>[7x]EVKQENRLLNESESSSQGLLGYYFSDLNFQAPMVVTSSTTGDLSIPSSELENIPSENQYFQSAIWSGFIKVKKSDEYTFATSADNHVTMWVDDQEVINKASNSNKIRLEKGRLYQIKIQYQRENPTEKGLDFKLYWTDSQNKKEVISSDNLQLPELKQKSSNSRKKRSTSAGPTVPDRDNDGIPDSLEVEGYTVDVKNKRTFLSPWISNIHEKKGLTKYKSSPEKWSTASDPYSDFEKVTGRIDKNVSPEARHPLVAAYPIVHVDMENIILSKNEDQSTQNTDSQTRTISKNTSTSRTHTSEVHGNAEVHASFFDIGGSVSAGFSNSNSSTVAIDHSLSLAGERTWAETMGLNTADTARLNANIRYVNTGTAPIYNVLPTTSLVLGKNQTLATIKAKENQLSQILAPNNYYPSKNLAPIALNAQDDFSSTPITMNYNQFLELEKTKQLRLDTDQVYGNIATYNFENGRVRVDTGSNWSEVLPQIQETTARIIFNGKDLNLVERRIAAVNPSDPLETTKPDMTLKEALKIAFGFNEPNGNLQYQGKDITEFDFNFDQQTSQNIKNQLAELNATNIYTVLDKIKLNAKMNILIRDKRFHYDRNNIAVGADESVVKEAHREVINSSTEGLLLNIDKDIRKILSGYIVEIEDTEGLKEVINDRYDMLNISSLRQDGKTFIDFKKYNDKLPLYISNPNYKVNVYAVTKENTIINPSENGDTSTNGIKKILIFSKKGYEIG;>MNEHYTESDIKRNHKTEKNKTEKEKFKDSINNLVKTEFTNETLDKIQQTQDLLKKIPKDVLEIYSELGGEIYFTDIDLVEHKELQDLSEEEKNSMNSRGEKVPFASRFVFEKKRETPKLIINIKDYAINSEQSKEVYYEIGKGISLDIISKDKSLDPEFLNLIKSLSDDSDSSDLLFSQKFKEKLELNNKSIDINFIKENLTEFQHAFSLAFSYYFAPDHRTVLELYAPDMFEYMNKLEKGGFEKISESLKKEGVEKDRIDVLKGEKALKASGLVPEHADAFKKIARELNTYILFRPVNKLATNLIKSGVATKGLNVHGKSSDWGPVAGYIPFDQDLSKKHGQQLAVEKGNLENKKSITEHEGEIGKIPLKLDHLRIEELKENGIILKGKKEIDNGKKYYLLESNNQVYEFRISDENNEVQYKTKEGKITVLGEKFNWRNIEVMAKNVEGVLKPLTADYDLFALAPSLTEIKKQIPQKEWDKVVNTPNSLEKQKGVTNLLIKYGIERKPDSTKGTLSNWQKQMLDRLNEAVKYTGYTGGDVVNHGTEQDNEEFPEKDNEIFIINPEGEFILTKNWEMTGRFIEKNITGKDYLYYFNRSYNKIAPGNKAYIEWTDPITKAKINTIPTSAEFIKNLSSIRRSSNVGVYKDSGDKDEFAKKESVKKIAGYLSDYYNSANHIFSQEKKRKISIFRGIQAYNEIENVLKSKQIAPEYKNYFQYLKERITNQVQLLLTHQKSNIEFKLLYKQLNFTENETDNFEVFQKIIDEK[2x]

Following assembly, the anthrax protective antigen (PA) forms an oligomeric translocon that unfolds and translocates either its lethal factor (LF) or edema factor (EF) into the host cell. The toxin functions as a binary A2B toxin, with enzymatic A factors, lethal factor (LF, 91 kDa) and edema factor (EF, 89 kDa), and a cell binding B factor, protective antigen (PA, 83 kDa). Within the endosomal compartment, the acidic environment induces a conformational change in the PA, resulting in the formation of a β-barrel channel that can insert itself into the endosomal membrane. The first α helix and β strand of LF and EF unfold and dock into a deep amphipathic cleft, called the α clamp, which resides at the interface of two PA monomers.

The available space on the heptameric PA channel for EF binding can only accommodate up to three EF molecules due to steric hindrance. Indeed, 2D classification of cryo-EM images of PA channel bound with EF showed that the EF binding varies in different classes, suggesting that the space is not fully occupied. Therefore, we used a symmetry expansion method in Relion for 3D classification and were able to resolve the asymmetrically attached EF. Unlike LF, all the domains of EF are well resolved in our channel complex structures. Upon PA binding, these disordered residues of EF (residues 20–30) refold into an α-helix (EFN α1) and bind within the α-clamp site. β1 (Leu33 to Lys35) of EFN forms parallel β-sheet with β13 (Leu203 to Pro205) of PAN. LF α1 is angled downward towards the pore in the α-clamp site, while the amino-terminal end of EF α1 is elevated ~2.9 Å as measured using the carbonyl groups on LF Glu34 and EF Glu24. This elevation in EF α1 appears to be caused by a change in the orientation of PAN Phe464. The phenyl ring in PAN Phe464 is positioned outwards toward the bound EF α1. This change in the orientation of Phe464 appears to restrict EF α1 in its elevated conformation in the α-clamp site. While in the PA7-bound EF structures, the HD domain contributes to a new conformation by bridging the PABD and ACD.> MEDLDERELKEAFRVLDKEKKGVIKVDVLRWILKSLGDELTEDEIENMIAETDTDGSGTVD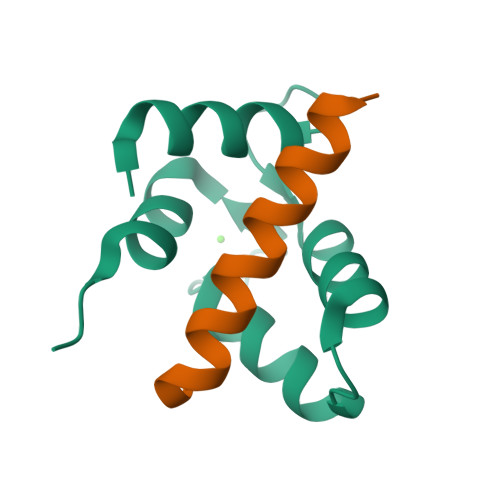YEEFKCLMMSSDA;> GLSPEKKKMLKKLIMQKAAEDLAN> SSLPVPYKLPVSLSVGSCVIIKGTPIHSFINGPQLQVDFYTDMDEDSDIAFHFNVRFGNHVVMNRREFGIWMLEETTDYVPFEDGKQFELCIYVHYNEYEIKVNGIRIYG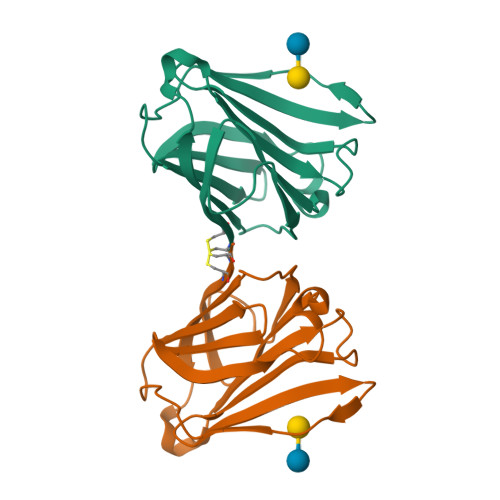FVHRIPPSFVKMVQVSRDISLTSVCVCN> MNGDCVDAKRVDTTDASKDGASASQPMQVDAKPQSHAFRYSLNYPNIGHCIIINNKNFDR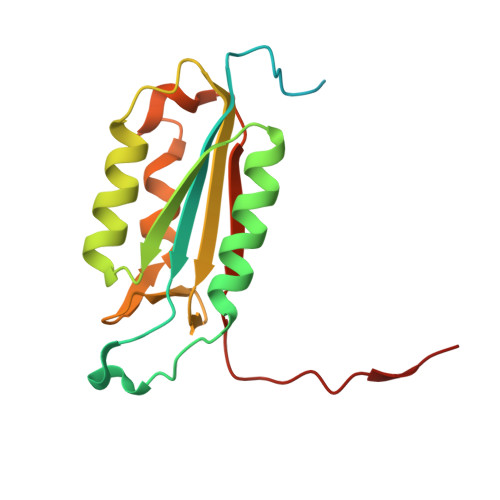RTGMNPRNGTDVDAGNVMNVFRKLGYIVKVYNDQTVAQIMQVLTTVAHDDHSRCASLVCVLLSHGDEGVFFGTDTSVDLKSLTSLFRGDRCPSLVGKPKLFFIQACRGTELDPGVETD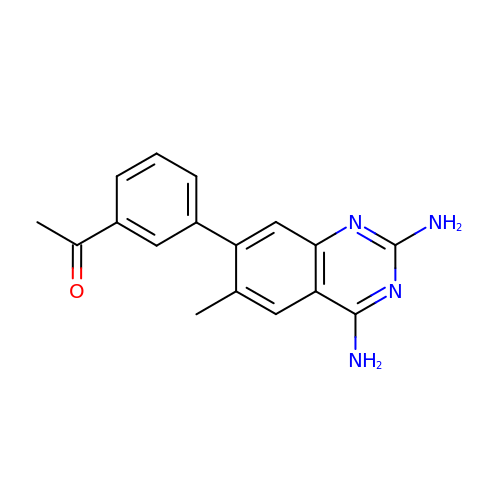1-[3-(2,4-diamino-6-methylquinazolin-7-yl)phenyl]ethanone | C17 H16 N4 O | OCMSAMCSELNFPL-UHFFFAOYSA-N> KRAALIQNLRDSYTETSSF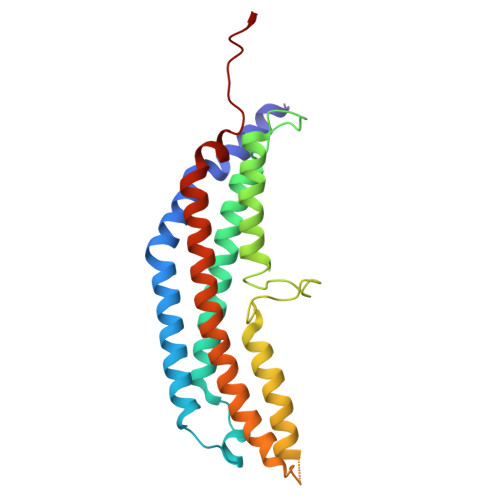AVIEEWAAGTLQEIEGIAKAAAEAHGVIRNSTYGRAQAEKSPEQLLGVLQRYQDLCHNVYCQAETIRTVIAIRIPEHKEEDNLGVAVQHAVLKIIDELEIKTLGSGEKSGSGGAPTPIGMYALREYLSARSTVEDKLLGSVDAESGKTKGGSQSPSLLLELRQIDADFMLKVELATTHLSTMVRAVINAYLLNWKKLIQPRTGTDHMFS>[2x]MSQSNRELVVDFLSYKLSQKGYSWSQMAAVKQALREAGDEFEL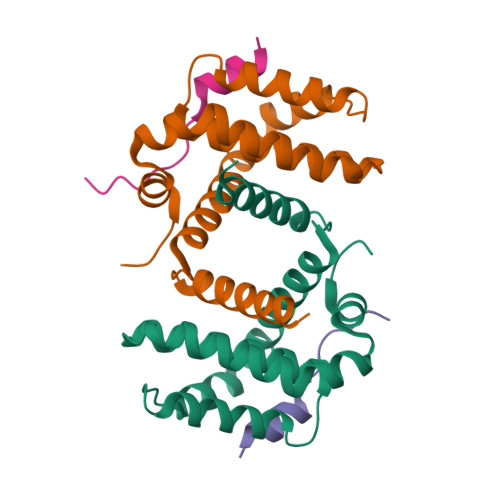RYRRAFSDLTSQLHITPGTAYQSFEQVVNELFRDGVNWGRIVAFFSFGGALCVESVDKEMQVLVSRIAAWMATYLNDHLEPWIQENGGWDTFVELYGNNAAAESRKGQER;>[2x]KDCVFKDWEELGEEIRLKVFVLG>MGFSADHSQIAQTKDTMFTGYLDPVQAKDYFAEAEKTSIVQRVAQKIPMGATGIVIPHWTGDVSAQWIGEGDMKPITKGNMTKRDVHPAKIATIFVASAETVRANPANYLGTMRTKVATAIAMAFDNAALHGTNAPSAFQGYLDQSNKTQSISPNAYQGLGVSGLTKLVTDGKKWTHTLLDDTVEPVLNGSVDANGRPLFVESTYESLTTPFREGRILGRPTILSDHVAEGDVVGYA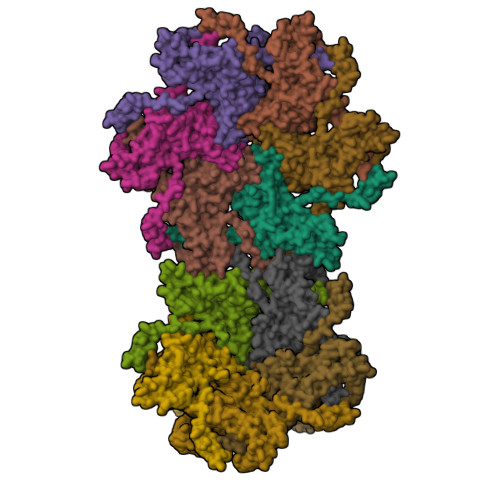GDFSQIIWGQVGGLSFDVTDQATLNLGSQESPNFVSLWQHNLVAVRVEAEYGLLINDVNAFVKLTFDPVLTTYALDLDGASAGNFTLSLDGKTSANIAYNASTATVKSAIVAIDDGVSADDVTVTGSAGDYTITVPGTLTADFSGLTDGEGASISVVSVG[11x]>MIPVTELRYFADTQPAYRILKPWWDVFTDYISIVMLMIAVFGGTLQVTQDKMICLPCKWVTKDSCNDSFRGWAASSPEPTYPNSTVLPTPDTGPTGIKYDLDRHQYNYVDAVCYENRLHWFAKYFPYLVLLHTLIFLACSNFWFKFPRTSSKLEHFVSILLKCFDSPWTTRALSETVVEESDPKPAFSKMNGSMDKKSSTVSEDVEATVPMLQRTKSRIEQGIVDRSETGVLDKKEGEQAKALFEKVKKFRTHVEEGDIVYRLYMRQTIIKVIKFALIICYTVYYVHNIKFDVDCTVDIESLTGYRTYRCAHPLATLFKILASFYISLVIFYGLICMYTLWWMLRRSLKKYSFESIREESSYSDIPDVKNDFAFMLHLIDQYDPLYSKRFAVFLSEVSENKLRQLNLNNEWTLDKLRQRLTKNAQDKLELHLFMLSGIPDTVFDLVELEVLKLELIPDVTIPPSIAQLTGLKELWLYHTAAKIEAPALAFLRENLRALHIKFTDIKEIPLWIYSLKTLEELHLTGNLSAENNRYIVIDGLRELKRLKVLRLKSNLSKLPQVVTDVGVHLQKLSI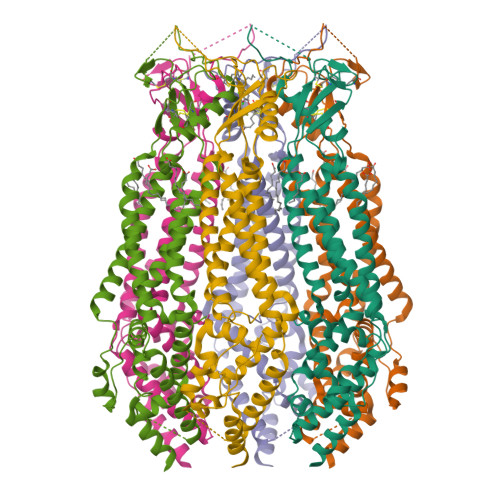NNEGTKLIVLNSLKKMVNLTELELIRCDLERIPHSIFSLHNLQEIDLKDNNLKTIEEIISFQHLHRLTCLKLWYNHIAYIPIQIGNLTNLERLYLNRNKIEKIPTQLFYCRKLRYLDLSHNNLTFLPADIGLLQNLQNLAVTANRIEALPPELFQCRKLRALHLGNNVLQSLPSRVGELTNLTQIELRGNRLECLPVELGECPLLKRSGLVVEEDLFSTLPPEVKERLWRADKEQASNSLEVLFQ[6x]>MVDVIALGEPLIQFNSFNPGPLRFVNYFEKHVAGSELNFCIAVVRNHLSCSLIARVGNDEFGKNIIEYSRAQGIDTSH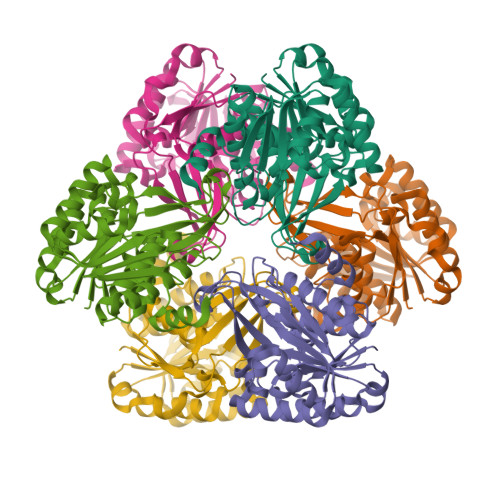IKVDNESFTGIYFIQRGYPIPMKSELVYYRKGSAGSRLSPEDINENYVRNSRLVHSTGITLAISDNAKEAVIKAFELAKSRSLDTNIRPKLWSSLEKAKETILSILKKYDIEVLITDPDDTKILLDVTDPDEAYRKYKELGVKVLLYKLGSKGAIAYKDNVKAFKDAYKVPVEDPTGAGDAMAGTFVSLYLQGKDIEYSLAHGIAASTLVITVRGDNELTPTLEDAERFLNEFKT[3x]> MAHHHHHHMAAFNTQKVLSVHHWTDAYFTFTCIRDESLRFENGQFVMVGLMADGKPLMRAYSVASANWEEHLEFFSIKVQDGPLTSRLQHLKVGDEVLISKKPTGTLVACDL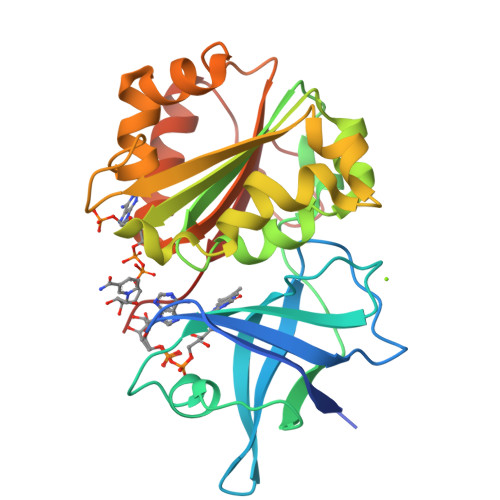NPGKHLYLLSTGTGIAPFLSITKDPEIYEQFEKIILVHGVRYKKDLAYYDRFTKELPEHEYLGDLVKEKLIYYPIVSREEFEHRGRLTDLMVSGKLFEDIGLPKINPQDDRAMLCGSPAMLKDTCKVLDDFGLTVSPKTGVRGDYLIERAFVDQ> MHHHHHHKNIINTSILSLRYENNHLIDLSRYASKINIGSRVNFDPIDKNQIQLFNLESSKIEVILKNAIVYNSMYENFSTSFWIKIPKYFSEISLNNEYTIINCIENNSGWKVSLNYGEIIWTLQDNKQNIQRVVFKYSQMVAISDYINRWIFITITNNRLTKSKIYINGRLIDQKPISNLGNIHASNKIMFKLDGCRDPRRYIMIKYFNLFDKELNEKEIKDLYDSQSNSGILKDFWGNYLQYDKPYYMLNLFDPNKYVDVNNVGIRGYMYLKGSRSTLLTTNIYLNSGLYMGTKFIIKKYASGNKDNIVRNNDRVYINVVVNNKEYRLATNASQAGVEKILSALEIPDIGNLSQVVVMKSKNDQGIRNKCKMNLQDNNGNDIGFIGFHKFNDIYKLVASNWYNRQIEISSRTFGCSWEFIPVDDGWGEKPL

Clostridium botulinum neurotoxin A (BoNT/A) targets the soluble N-ethylmaleimide-sensitive factor attachment protein receptor (SNARE) complex, by cleaving synaptosomal-associated protein of 25 kDa size (SNAP-25). The HC, which consists of an N-terminal (HCN) and a C-terminal (HCC) subdomain, is responsible for BoNT’s high target specificity where it forms a dual-receptor complex with synaptic vesicle protein 2 (SV2) and a ganglioside receptor on the surface of motor neurons. Here, we report the high-resolution structure of BoNT/A6 cell binding domain in complex with GD1a (HC/A6:GD1a), and a new crystal form of HC/A6 [HC/A6 (crystal form II)]. A detailed analysis of these two structures along with a previous HC/A6 structure [HC/A6 (crystal form I)], reveals the interactions that occur across the HC/A6:GD1a interface, and the conformational flexibility of HC/A6.

The crystal structure of HC/A6:GD1a complex was determined at 1.5 Å resolution by molecular replacement in the monoclinic space group P21 with one molecule in the asymmetric unit. There was clear electron density at the expected ganglioside binding site (GBS) for which 5 out of the 6 GD1a monosaccharides could be modelled (blue). Furthermore, HC/A6 forms seven hydrogen bonds with GD1a at Sia5, Gal4, and GalNAc3 through six residues that are conserved among all BoNT/A subtypes. The HC/A6:GD1a interface is most similar to HC/A5, forming a total of 7 hydrogen bonds with the three monosaccharides GalNAc3, Gal4 and Sia5. Overall, the conformation of HC/A6 upon binding GD1a does not change dramatically except for a flipping of the Phe 1278 sidechain towards Sia5 of GD1a and an accompanying widening of loop 1269–1277. However, at the GBS, residue Phe 1278 rotates towards Sia5 and the loop 1269–1277 appears to widen by 4 Å (measured by the difference in Cα position between Arg 1269 and Thr 1277 residues) (magenta). This was observed previously for HC/A2, HC/A3, and HC/A5. The first is within the SV2 binding site (1139–1157) where residues 1150–1152 in both HC/A6:GD1a and HC/A6 (crystal form I) structures form a β-sheet with residues 1003–1006. For the HC/A6 (crystal form II) structure there is a continuation of electron density between the Nζ of Lys 1236 and Sγ of Cys 1280 residues, whereas in the HC/A6:GD1a structure Cys 1280 forms a disulphide bridge with Cys 1236, and the structure of HC/A6 (crystal form I) shows neither (blue). The raw plot shows higher B-factors overall for the HC/A6 (crystal form II) structure, indicating more flexibility across the entire molecule compared to the HC/A6:GD1a structure. For the latter, the HCC subdomain is more flexible than the HCN.>MLHILCQGTPFEIGYEHGSAAKAVIARSIDFAVDLIRGKTKKTDEELKQVLSQLGRVIEERWPKYYEEIRGIAKGAERDVSEIVMLNTRTEFAYGLKAARDGCTTAYCQLPNGALQGQNWDFFSATKENLIRLTIRQAGLPTIKFITEAGIIGKVGFNSAGVAVNYNALHLQGLRPTGVPSHIALRIALESTSPSQAYDRIVEQGGMAASAFIMVGNGHEAFGLEFSPTSIRKQVLDANGRMVHTNHCLLQHGKNEKELDPLPDSWNRHQRME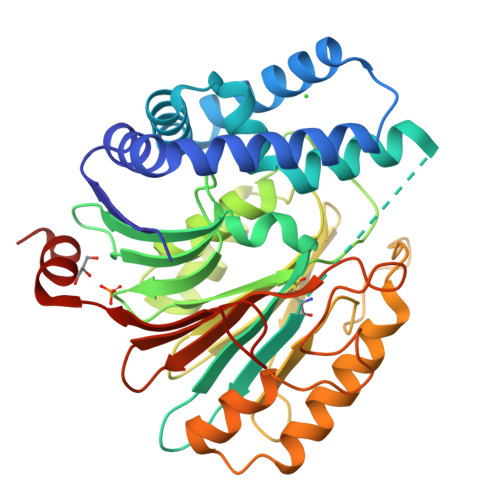FLLDGFDGTKQAFAQLWADEDNYPFSICRAYEEGKSRGATLFNIIYDHARREATVRLGRPTNPDEMFVMRFDEEDERSALNARL[4x]NEXTURASTAT A | C19 H23 N3 O3 | 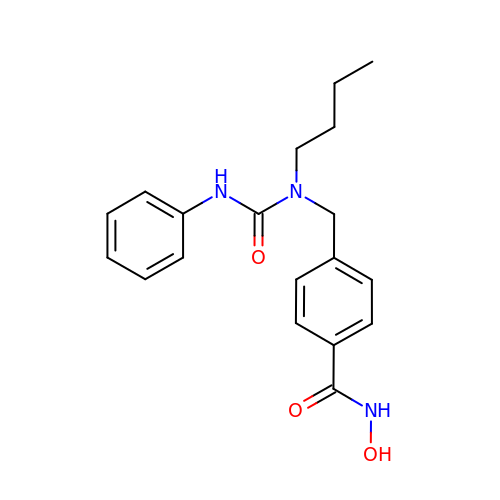JZWXMCPARMXZQV-UHFFFAOYSA-N>MGEEEESLAILRRHVMNELLDTERAYVEELLCVLEGYAAEMDNPLMAHLISTGLQNKKNILFGNMEEIYHFHNRIFLRELESCIDCPELVGRCFLERMEEFQIYEKYCQNKPRSESLWRQCSDCPFFQECQKKLDHKLSLDSYLLKPVQRITKYQLLLKEMLKYSKHCEGAEDLQEALSSILGILKAVNDSMHLIAITGYDGNLGDLGKLLMQGSFSVWTDHKKGHTKVKELARFKPMQRHLFLHEKAVLFCKKREENGEGYEKAPSYSYKQSLNMTAVGITENVKGDTKKFEIWYNAREEVYIIQAPTPE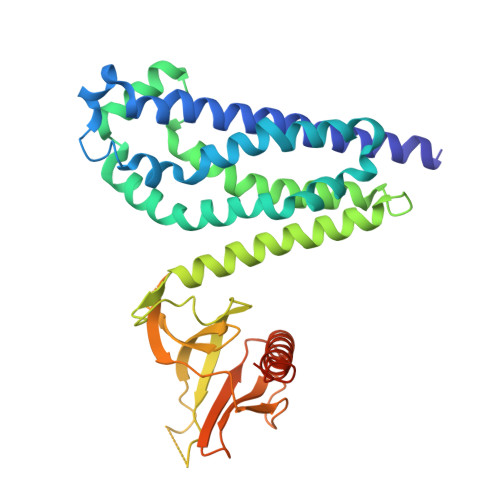IKAAWVNEIRKVLTSQLQACREASQHRALEQSHSLPHHHHHH[4x]>[2x]MPLDPQIKPILERIRALSIAASPQELRRQVEEQSRLLTAAVQEPIAETRDVHIPVSGGSIRARVYFPKKAAGLPAVLYYHGGGFVFGSIETHDHICRRLSRLSDSVVVSVDYRLAPEYKFPTAVEDAYAALKWVADRADELGVDPDRIAVAGDSAGGNLAAVVSILDRNSGEKLVKKQVLIYPVVNMTGVPTASLVEFGVAETTSLPIELMVWFGRQYLKRPEEAYDFKASPLLADLGGLPPALVVTAEYDPLRDEGELYAYKMKASGSRAVAVRFAGMVHGFVSFYPFVDAGREALDLAAASIRSGLQPS

EstE1 is a hyperthermophilic esterase belonging to the hormone-sensitive lipase family and was originally isolated by functional screening of a metagenomic library constructed from a thermal environmental sample. EstE1 is composed of 311 amino acid residues with a calculated molecular weight of approximately 34 kDa. EstE1 has a characteristic α/β hydrolase fold with nine alpha helices and an eight-stranded β-sheet. The residues Ser154, Asp251, and His281 of the catalytic triad are found in the canonical positions observed in a wide variety of α/β hydrolases.

The 2.1-Å resolution crystal structure of the selenomethionine derivative of EstE1 was determined in space group P41212 (unit cell dimensions of a = b = 73.71 Å, c = 234.23 Å, and α = β = γ = 90°) with two independent molecules per asymmetric unit, by single wavelength anomalous dispersion (SAD) method. The final structure of EstE1 displayed a nearly ellipsoidal shape with approximate dimensions of 46 Å × 47 Å × 57 Å. The electron density of the N-terminal 16 residues, which is expected to include the α1 (Lys8-Arg13) helix, was disordered. The cap domain consists of two separated helical regions (containing residues 1–41 and 193–218) and locates to the upper region of the central β-sheet. The substrate-binding pocket of EstE1 extends approximately 16 Å from the protein surface to the catalytic Ser154 residue. The sequence motif His-Gly-Gly-Gly (residues 80–83), which is conserved in the HSL family, is upstream of the active site. It is involved in hydrogen bonding for stabilization of the oxyanion hole formed by Gly82, Gly83, and Ala155. EstE1 dimerization is primarily mediated by hydrophobic interactions in the middle of the interface and is assisted by salt bridges at both ends of the interface. The dimeric interface is characterized by the formation of β-sheet between the two monomers by an antiparallel association between two C-terminal β8 strands. We also identified hydrophobic interactions between Val274 (on the β8 strand), Phe276 (on the β8 strand), and Leu299 (on the α9 helix). Site-directed mutagenesis analysis revealed that hydrophobic interactions through Val274 and Phe276 on the β8 strand at dimer interface contribute to the formation of EstE1 dimers and their hyperthermostability.6-[4-(dimethylamino)but-1-yn-1-yl]-4-methylpyridin-2-amine 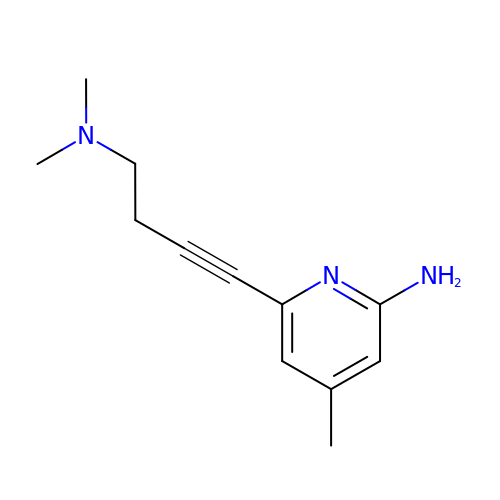| C12 H17 N3 | SWAXYJVGMJZMLB-UHFFFAOYSA-N>DDAAIQQTLAKMGIKSSDIQPAPVAGMKTVLTNSGVLYITDDGKHIIQGPMYDVSGTAPVNVTNKMLLKQLNALEKEMIVYKAPQEKHVITVFTDITCGYSHKLHEQMADYNALGITVRYLAFPRQGLDSDAEKEMKAIWCAKDKNKAFDDVMAGKSVAPASCDVDIADHYALGVQLGVSGTPAVVLSNGTLVP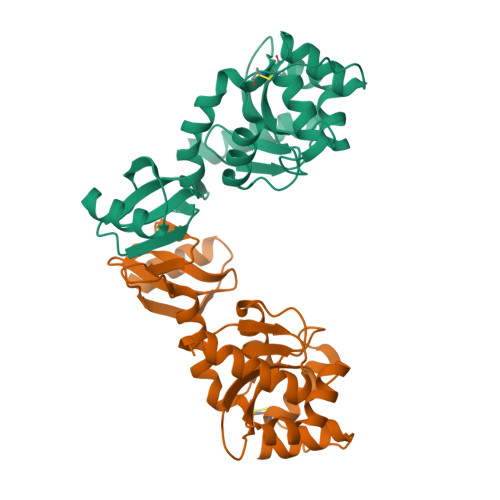GYQPPKEMKEFLDEHQKMTSGK[2x]>[6x]MNYWIAATGALALAVAVTAQGTTLLHNAKAQVTTPCGASHYMRHITRQAESALQAGLKTAQSALETSNKLRVVASSKTGGAATAASILAANLASEAAKAIETIKTETKNFLAGFAAAAELAGQQTIVSEIKSAQVQDVNTLTAAQAVTTPGIIQVKPKLTIASTAACFNDDGSPVSDDEAAQPNQGEPTLKFFVVSANTPGTTHNELLTICGHGSTGTAPSTGCQNDATSI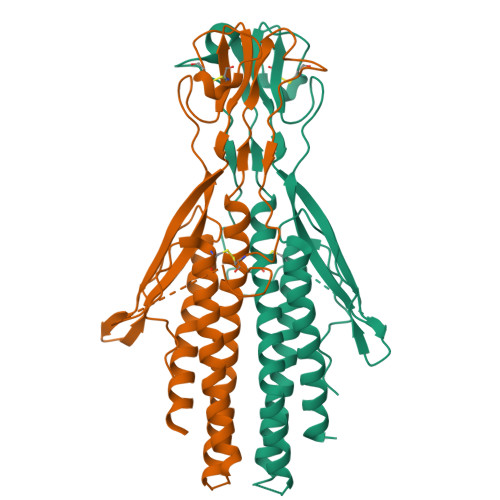GIKGGDFLKTAAVTTTRLASSAGKTYPAITSTTTIPNDKTLNKAVTAIRELETAVAALDAISDVSSPEDIAARPELTEAIAKALDGDKAKVDSFAAETFGKESAIVKSTIVKDLKDLKPPKSAVGGSGEKKLETINDPKELADAQIYYTVKKFVDEQEQKKKNQASPSCPTNTDKTTEPAKSADECKKHTTSDDCKDEKGCEFDEKKDPKCFPKVDTEKKDDKSFSSNVRVSVPQVFAALVLAAF> MKVRVKAPCTSANLGVGFDVFGLCLKEPYDVIEVE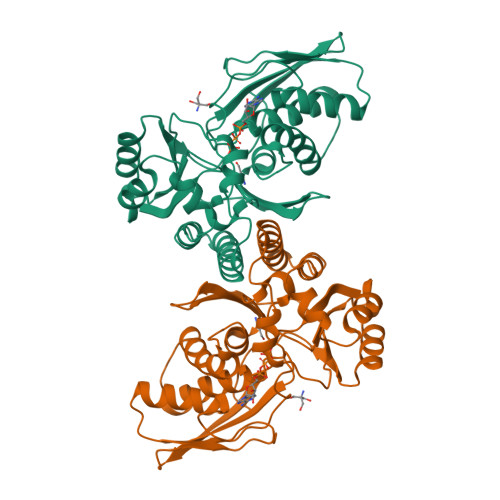AIDDKEIIIEVDDKNIPTDPDKNVAGIVAKKMIDDFNIGKGVKITIKKGVKAGSGLGSSAASSAGTAYAINELFKLNLDKLKLVDYASYGELASSGAKHADNVAPAIFGGFTMVTNYEPLEVLHIPIDFKLDILIAIPNISINTKEAREILPKAVGLKDLVNNVGKACGMVYALYNKDKSLFGRYMMSDKVIEPVRGKLIPNYFKIKEEVKDKVYGITISGSGPSIIAFPKEEFIDEVENILRDYYENTIRTEVGKGVEVV>[2x]SAPRESPLPYHIPLDPEGSLELSWNVSYTQEAIHFQLLVRRLKAGVLFGMSDRGELENADLVVLWTDGDTAYFADAWSDQKGQIHLDPQQDYQLLQVQRTPEGLTLLFKRPFGTCDPKDYLIEDGTVHLVYGILEEPFRSLEAINGSGLQMGLQRVQLLKPNIPEPELPSDACTMEVQAPNIQIPSQETTYWCYIKELPKGFSRHHIIKYEPIVTKGNEALVHHMEVFQCAPEMDSVPHFSGPCDSKMKPDRLNYCRHVLAAWALGAKAFYYPEEAGLAFGGPGSSRYLRLEVHYHNPLVIEGRN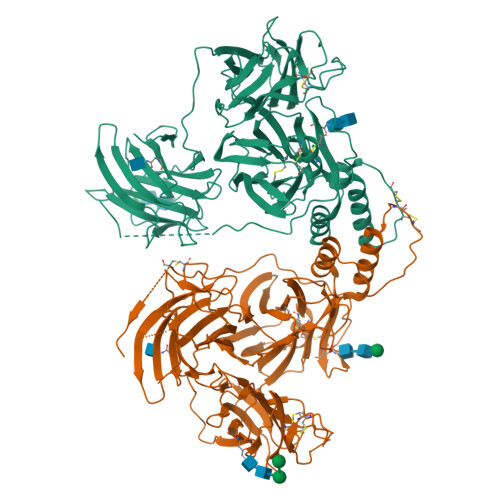DSSGIRLYYTAKLRRFNAGIMELGLVYTPVMAIPPRETAFILTGYCTDKCTQLALPPSGIHIFASQLHTHLTGRKVVTVLVRDGREWEIVNQDNHYSPHFQEIRMLKKVVSVHPGDVLITSCTYNTEDRELATVGGFGILEEMCVNYVHYYPQTQLELCKSAVDAGFLQKYFHLINRFNNEDVCTCPQASVSQQFTSVPWNSFNRDVLKALYSFAPISMHCNKSSAVRFQGEWNLQPLPKVISTLEEPTPQCPTSQGRSPAGPTVVSIGGGKG>[2x]MSRLAEFAAAEKALQEQMAQLEALKKDAGLKREIEFEQKLVGLMKSYDKSL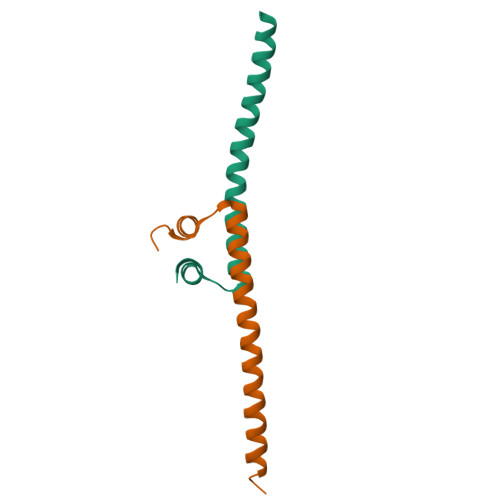RDIIAILDPKLEHHHHHH> GHHHHHHHGESLFKGPRDYNPISSTICHLTNESDGHTTSLYGIGFGPFIITNKHLFRRNNGTLLVQSLHG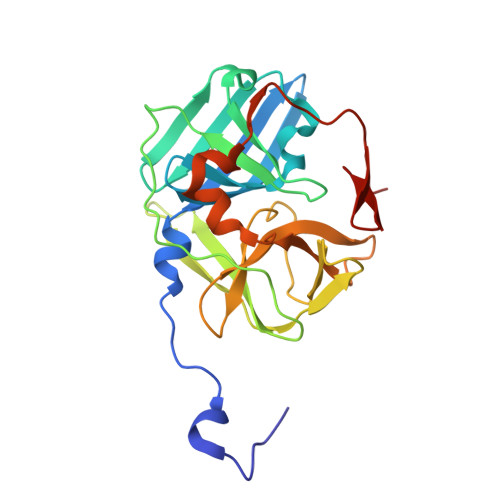VFKVKNTTTLQQHLIDGRDMIIIRMPKDFPPFPQKLKFREPQREERICLVTTNFQTKSMSSMVSDTSCTFPSSDGIFWKHWIQTKDGQCGSPLVSTRDGFIVGIHSASNFTNTNNYFTSVPKNFMELLTNQEAQQWVSGWRLNADSVLWGGHKVFMDKP> GFPCGESCVYIPCFTAAIGCSCKSKV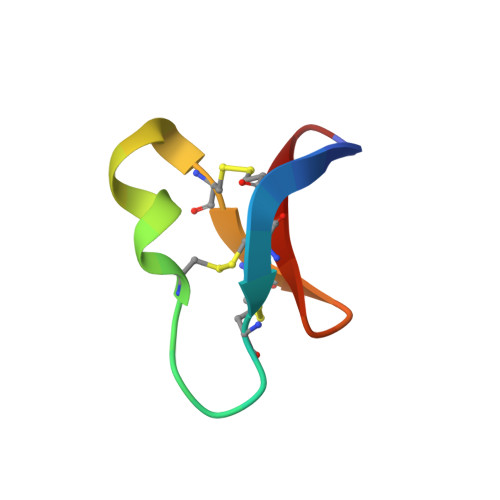CYKN>MEYSD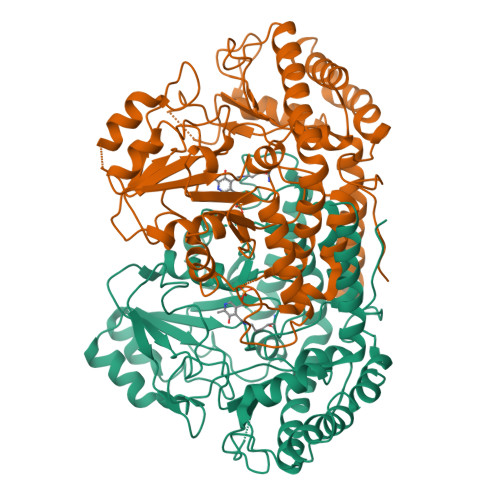VPKFIRDVSIKQHEWMRESIKLIASENITSLAVREACATDFMHRYAEGLPGKRLYQGCKYIDEVETLCIELSKELFKAEHANVQPTSGVVANLAVFFAETKPGDKLMALSVPDGGHISHWKVSAAGIRGLKVINHPFDPEEMNIDADAMVKKILEEKPKLILFGGSLFPFPHPVADAYEAAQEVGAKIAYDGAHVLGLIAGKQFQDPLREGAEYLMGSTHKTFFGPQGGVILTTKENADKIDSHVFPGVVSNHHLHHKAGLAIALAEMLEFGEAYAKQVIKNAKALAQALYERGFNVLCEHKDFTESHQVIIDIESSPDIEFSASELAKMYEEANIILNKNLLPWDDVNNSDNPSGIRLGTQECTRLGMKEKEMEEIAEFMKRIAIDKEKPEKVREDVKEFAKEYSTIHYSFDEGDGFKYLRFY[12x]>MTTFLIKHKASGKFLHPKGGSSNPANDTNLVLHSDIHERMYFQFDVVDERWGYIKHAASGKIVHPLGGKADPPNETKLVLHQDRHDRALFAMDFFNDNIIHKAGKYVHPKGGSTNPPNETLTVMHGDKHGA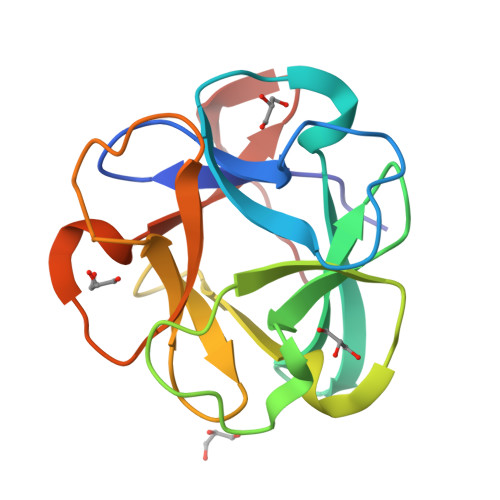MEFIFVSPKNKDKRVLVYV[2x]> MLKQVEIFTDGSCLGNPGPGGYAAILRYRGREKTFSAGYTRTTNNRMELMAAIVALEALKEPCEVILSTDSQYLRQGITQWIHNWKKRGWKTADGKPVKNVDLWQRL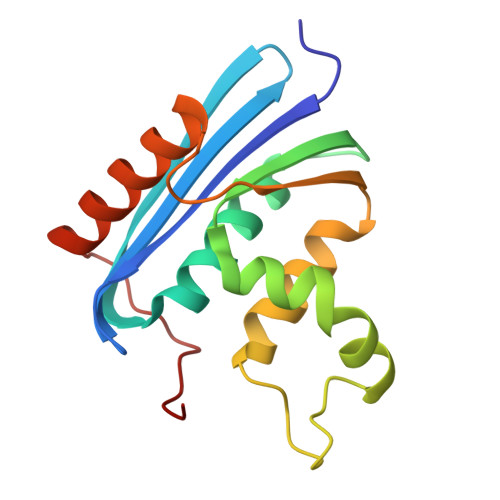DAALGQHQIKWEWVKGHAGHPENERCHELARAAAMNPTLEDTGYQVEV(1-propylpyrazol-4-yl)methyl 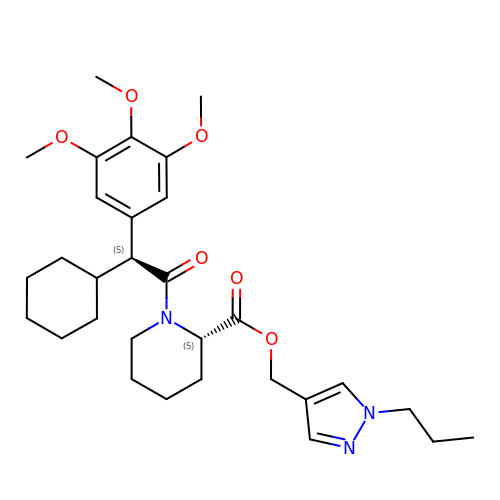(2S)-1-[(2S)-2-cyclohexyl-2-(3,4,5-trimethoxyphenyl)ethanoyl]piperidine-2-carboxylate | C30 H43 N3 O6 | HVWPRXIQGCFSII-IGKIAQTJSA-N>GMREMQIMSQPEQSRLDLFIDRMVSQRACLEHAIAQTAGLSGPVYELGLGNGRTYHHLRQHVQGREIYVFERAVASHPDSTPPEAQLILGDIRETLPATLERFGATASLVHADLGGHNREKNDRFARLISPLIEPHLAQGGLMVSSDRMYFEGLEELPLPPGAVV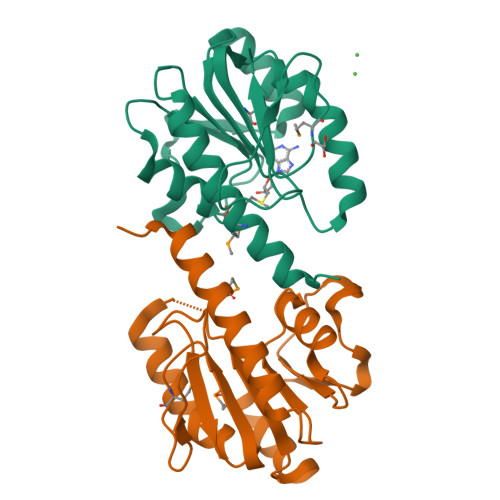GRCFIYRRG[2x]>[2x]GPLGSDHKEPEIITVTLKKQNGMGLSIV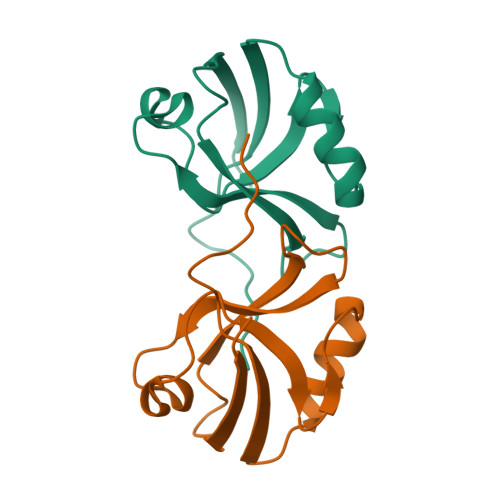AAKGAGQDKLGIYVKSVVKGGAADVDGRLAAGDQLLSVDGRSLVGLSQERAAELMTRTSSVVTLEVAKQGAIRREWYV> MSSTKCAVACKIMTPLCNAASKVQARSAKKLAALTDAGIQKTISEHNANGTDAAVSSTKRYLAEQRQLFH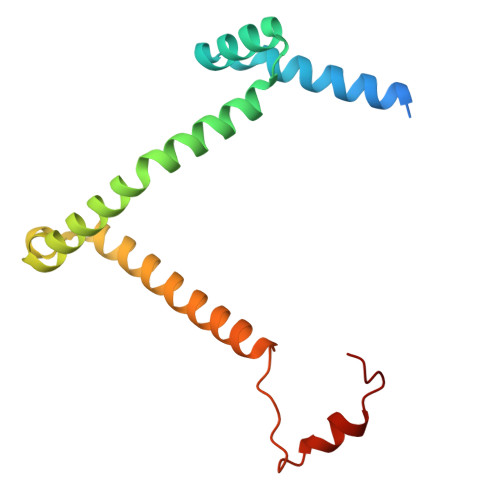YRVVRFFDECHYIISGEYFAQYTKVNLIWDLRFLTKLVVLFLIGTVLGRQSIFPPIDPDSPLVEALVTKVNPNY>[2x]HGYVSAVENGVAEGRVTLCKFAANGTGEKNTHCGAIQYEP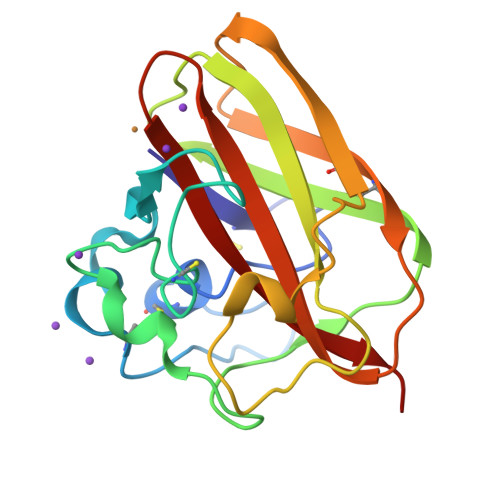QSVEGPDGFPVTGPRDGKIASAESALAAALDEQTADRWVKRPIQAGPQTFEWTFTANHVTKDWKYYITKPNWNPNQPLSRDAFDLNPFCVVEGNMVQPPKRVSHECIVPEREGYQVILAVWDVGDTAASFYNVIDVKFDG> MIITSPTEARKDFYQLLKNVNNNH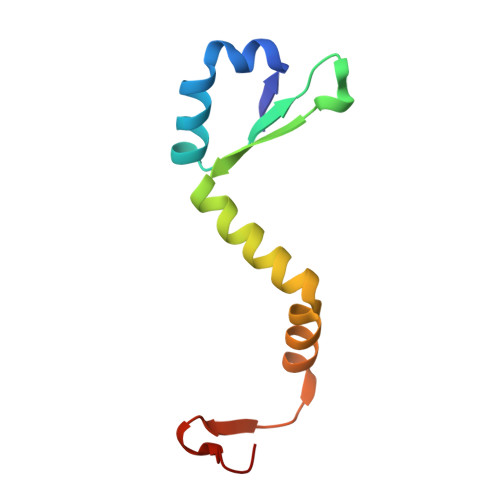EPIYISGNNAENNAVIIGLEDWKSIQETIYLESTGTMDKVREREKDNSGTTNIDDIDWDNL> MSLAFYIATFDIGTTEVKAALADRDGGLHFQRSIALETYGDGNGPVEQDAGDWYDAVQRIASSWWQSGVDARRVSAIVLSGQMQNFLPLDQDHEPLHRAVLYSDKRPLKEAEEINAR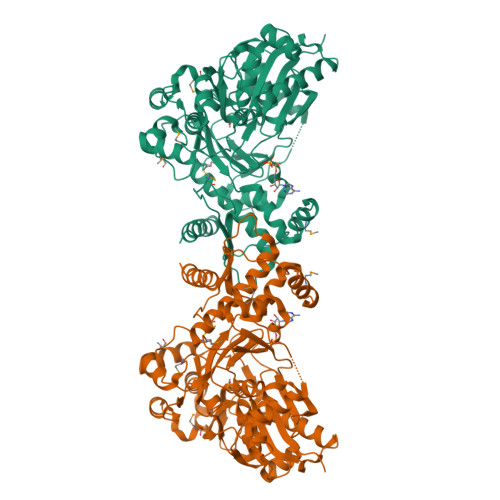HGADNLWSALENPMTAASILPKLVFWRASFPQAFGRLRHVVLGAKDYVVLRLTGRHATDRTNASTTGLYRPKDDAWHVELLADYGFSLDLMPRLLEPGEQVGGVSALAARQTGFVSGTPVLCGLGDAGAATLGVGVLDDEDAYLHLGTTGWLARLTQTDPVGDMPVGTIFRLAGIIAGKTLQVAPVLNAGNILQWALTLVGHRPGEDCAEYFHMAAAEVQGVTVPDGLLFVPYLHAERCPVELPAPRGALLGVTGATTRAQILLAVLEGAALSLRWCAELLGMEKVGLLKVVGGGARSEAWLRMIADNLNVSLLVKPDAHLHPLRGLAALAAVELEWSHSIQDFLREADLREPASNILHPQPCDEGRRRRKFERFKQCVETLGRLDEGHHHHHH> MRSVTNAFGNSGELNDQVDETGYRKFDIHEGILFCIELSETMFKESSDLEYKSPLLEILESLDELMSQLVITRPGTAIGCYFYYCNREDAKEGIYELFPLRDINATFMKKLNDLLEDLSSGRISLYDYFMFQQTGSEKQVRLSVLFTFMLDTFLEEIPGQKQLSNKRVFLFTDIDKPQEAQDIDERARLRRLTIDLFDNKVNFATFFIGYADKPFDNEFYSDILQLGSHTNENTGLDSEFDGPSTKPIDAKYIKSRILRKKEVKRIMFQCPLILDEKTNFIVGVKGYTMYTHEKAGVRYKLVYEHEDIRQEAYSKRKFLNPITGEDVTGKTVKVYPYGDLDINLSDSQDQIVMEAYTQKDAFLKIIGFRSSSKSIHYFNNIDKSSFIVPDEAKYEGSIRTLASLLKILRKKDKIAILWGKLKSNSHPSLYTLSPSSVKDYNEGFYLYRVPFLDEIRKFPSLLSYDDGSEHKLDYDNMKKVTQSIMGYFNLRDGYNPSDFKNPLLQKHYKVLHDYLLQIETTFDENETPNTKKDRMMREDDSLRKLYYIRNKILESEKSEDPIIQRLNKYVKIWNMFYKKFNDDNISIKEEKKPFDKKPKFNI;> MSSESTTFIVDVSPSMMKNNNVSKSMAYLEYTLLNKSKKSRKTDWISCYLANCPVSENSQEIPNVFQIQSFLAPVTTTATIGFIKRLKQYCDQHSHDSSNEGLQSMIQCLLVVSLDIKQQFQARKILKQIVVFTDNLDDLDITDEEIDLLTEELSTRIILIDCGKDTQEERKKSNWLKLVEAIPNSRIYNMNELLVEITSPATSVVKPVRVFSGELRLGADILSTQTSNPSGSMQDENCLCIKVEAFPATKAVSGLNRKTAVEVEDSQKKERYVGVKSIIEYEIHNEGNKKNVSEDDQSGSSYIPVTISKDSVTKAYRYGADYVVLPSVLVDQTVYESFPGLDLRGFLNREALPRYFLTSESSFITADTRLGCQSDLMAFSALVDVMLENRKIAVARYVSKKDSEVNMCALCPVLIEHSNINSEKKFVKSLTLCRLPFAEDERVTDFPKLLDRTTTSGVPLKKETDGHQI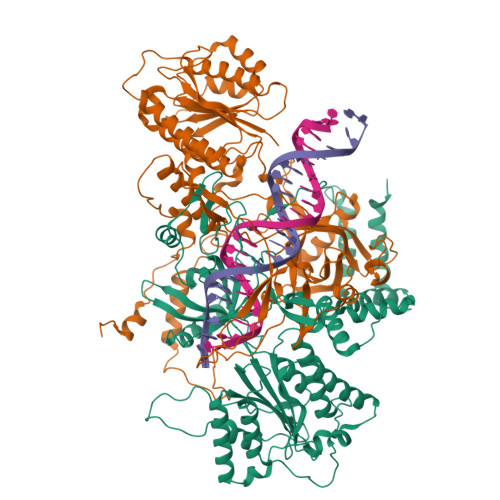DELMEQFVDSMDTDELPEIPLGNYYQPIGEVTTDTTLPLPSLNKDQEENKKDPLRIPTVFVYRQQQVLLEWIHQLMINDSREFEIPELPDSLKNKISPYTHKKFDSTKLVEVLGIKKVDKLKLDSELKTELEREKIPDLETLLKRGEQHSRGSPNNSNN Here, we describe identification of two bacterial effectors that reverse PR ubiquitination and are thus named deubiquitinases for PR ubiquitination (DUPs; DupA and DupB). Structural analyses revealed that DupA and SidE ubiquitin ligases harbor a highly homologous catalytic phosphodiesterase (PDE) domain. However, unlike SidE ubiquitin ligases, DupA displays increased affinity to PR-ubiquitinated substrates, which allows DupA to cleave PR ubiquitin from substrates.

The overall structure of DupA resembled the PDE domains of the SidE family ligases SdeA (Kalayil et al., 2018) and SidE (Wang et al., 2018) as well as the PDE domain of DupB (Akturk et al., 2018). The three catalytic residues from SdeA and DupB PDE domains were also highly conserved in the core of DupA (H67, E126, and H189), while several loop regions differed. Varying the length of the corresponding SdeA loop, deleting the loop regions from both SdeA and DupA PDE domains, or swapping the loop region did not affect the function of either PDE domains. In contrast, mutation of the three conserved catalytic residues from both DupA and DupB resulted in impaired cleavage activity. Moreover, after 5 min of reaction, we detected a labile and heat-sensitive His-Ub intermediate on the DupA His-189-Asn mutant, while wild-type (WT) DupA displayed heat-stable auto-PR ubiquitination , which was further cleaved by DupA at later time points. This suggests that, similar to the SdeA PDE domain, DupA utilizes a histidine-based intermediate reaction to catalyze the hydrolysis of ADPR-Ub (Kalayil et al., 2018). Thus, the PDE domains of SidEs and DupA/B may share the same catalytic residues to mediate opposite reactions: PR-Ub transfer to substrates and removal of PR-Ub from substrates (deubiquitination), respectively.

> SILDPEVLKVAEYVYQERLSKPYTEVGPEWEYNHKTPYATRATGTGHNLQRFITIDDQRLHRPIHGLAHTMRTLFYSQLMYEAAKRQPHPHRCADGRTIADLSVQDLKKLNIAQLFFVAGRESEASYGDAYHRYHLYGAKQFEAYARKHLTHLFSEKEIVLYSRCIEDRIGDRFDETAEGYLIHLSHMIDLMRCKSPVEVFIGHSRGVSGIVPTLIQLFGREDGLDIMHYARSLFAATGEAVPYISSSEWPHLGIESDRVERALKIVGSLEVEGQEADAKKTAQAGFSVDGCYGALVKIDTPDWYHQVKEKEDYDVDEVIALPPQITIREEPPKTNESFLLSL;> GSILDPEVLKVAEYVYQERLSKPYTEVGPEWEYNHKTPYATRATGTGHNLQRFITIDDQRLHRPIHGLAHTMRTLFYSQLMYEAAKRQPHPHRCADGRTIADLSVQDLKKLNIAQLFFVAGRESEASYGDAYHRYHLYGAKQFEAYARKHLTHLFSEKEIVLYSRCIEDRIGDRFDETAEGYLIHLSHMIDLMRCKSPVEVFIGHSRGVSGIVPTLIQLFGREDGLDIMHYARSLFAATGEAVPYISSSEWPHLGIESDRVERALKIVGSLEVEGQEADAKKTAQAGFSVDGCYGALVKIDTPDWYHQVKEKEDYDVDEVIALPPQITIREEPPKTNESFLLSL;> GAMGSILDPEVLKVAEYVYQERLSKPYTEVGPEWEYNHKTPYATRATGTGHNLQRFITIDDQRLHRPIHGLAHTMRTLFYSQLMYEAAKRQPHPHRCADGRTIADLSVQDLKKLNIAQLFFVAGRESEASYGDAYHRYHLYGAKQFEAYARKHLTHLFSEKEIVLYSRCIEDRIGDRFDETAEGYLIHLSHMIDLMRCKSPVEVFIGHSRGVSGIVPTLIQLFGREDGLDIMHYARSLFAATGEAVPYISSSEWPHLGIESDRVERALKIVGSLEVEGQEADAKKTAQAGFSVDGCYGALVKIDTPDWYHQVKEKEDYDVDEVIALPPQITIREEPPKTNESFLLSL>TIQGSIVAIVTPMLKDGGVDWKSLEKLVEWHIEQGTNSIVAVGTTGEASTLSMEEHTQVIKEIIRVANKRIPIIAGTGANSTREAIELTKAAKDL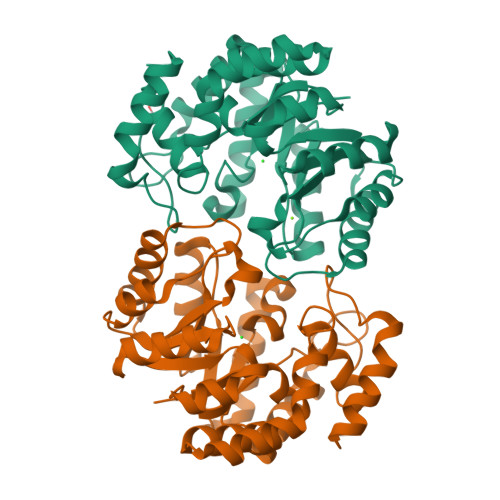GADAALLVTPYYNKPTQEGLYQHYKAIAEAVELPLILYNVPGRTGVDLSNDTAVRLAEIPNIVGIKDATGDVPRGKALIDALNGKMAVYSGDDETAWELMLLGADGNISVTANIAPKAMSEVCAVAIAKDEQQAKTLNNKIANLHNILFCESNPIPVKWALHEMGLIDTGIRLPLTPLAEQYREPLRNALKDAGII[2x]>MNKTYAACSKNWTGVGNKCFYFSGYPRNWTFAQAFCMAQEAQLARFDNEEELIFLKRFKGDFDSWIGLHRESSEHPWKW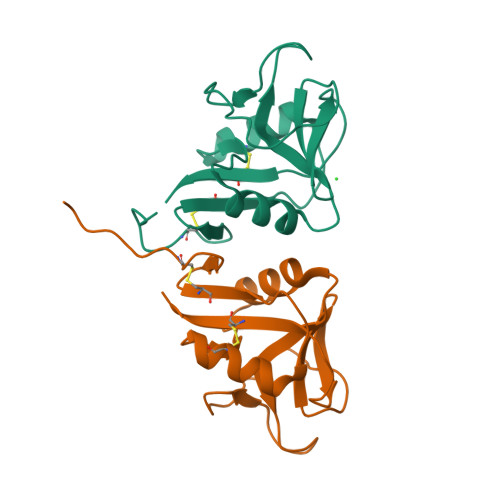TNNTEYNNMNPILGVGRYAYLSSDRISSSRSYINRMWICSKLN[2x]>[14x]MNLIPTVIETTNRGERAYDIYSRLLKDRIIMLGSQIDDNVANSIVSQLLFLQAQDSEKDIY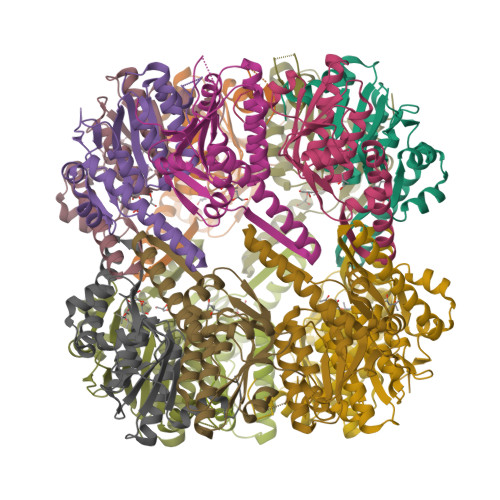LYINSPGGSVTAGFAIYDTIQHIKPDVQTICIGMAASMGSFLLAAGAKGKRFALPNAEVMIHQPLGGAQGQATEIEIAANHILKTREKLNRILSERTGQSIEKIQQDTDRDNFLTAAEAKEYGLIDEVMEPEHHHHHH L-gamma-glutamyl-L-alanylglycine | C10 H17 N3 O6 | 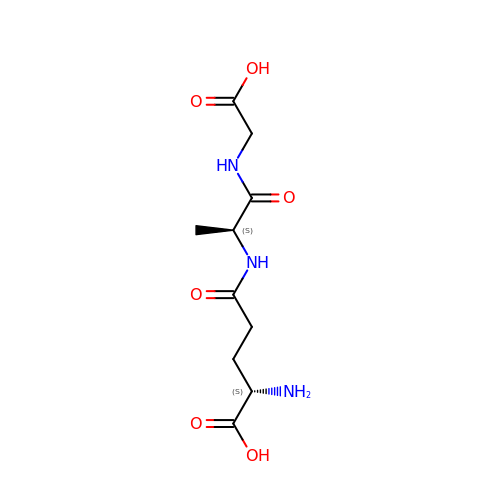RPVCUZZJCXVVDW-WDSKDSINSA-N> GAMGKSEGVTIEFKIVGLNKKLKVFTTCPHTLFGASFCAVAIEHPIVQDLMSKEIQDLISSIKIQGKNNEKVGIYTGLNVKHPFLDKELPLYVANFVLMEYREGAIFGCPAHDQRDFEFAQEYDLPIIPVISSARLGIEEYTNNSIMFNSEFLNGLTVSEARKVIVEK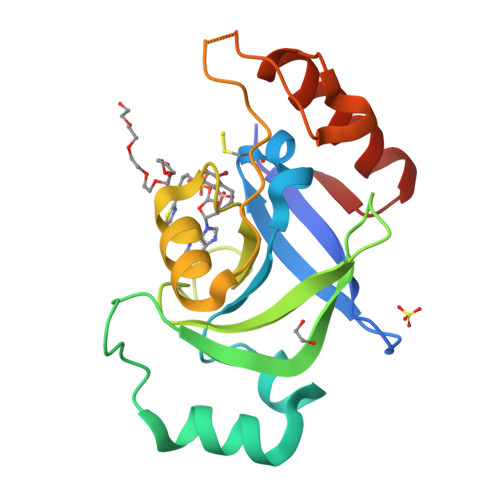LEEKGIGKKTI Using an X-ray free electron laser (XFEL), we have previously determined room-temperature (RT) serial femtosecond crystallography (SFX) structures of the ferric and Compound I redox states of DtpB,26 a B-type member of the dye-decolorizing peroxidase (DyP) family. Such an approach results in “pristine” DtpB structures that do not exhibit the effects of X-ray-generated radiation damage. The RT-SFX DtpB ferric and Compound I structures revealed that the distal heme pocket, which is composed of an Asp–Arg–Asn triad, was void of H2O molecules. DtpB, therefore, represents an exemplar of a His–heme-ligated peroxidase in which the distal heme pocket favors a dry site. By disrupting the distal heme pocket Asp–Asn–Arg triad in DtpB, our RT-SFX structures reveal that a wet site can be formed.

To assess whether disruption of the Asp–Arg–Asn triad in DtpB leads to a wet distal heme pocket, microcrystals of each variant in the Fe(III)–heme state were produced and subjected to RT-SFX crystallography using a high viscosity extruder sample delivery system at the SACLA XFEL beamline BL2 EH3. For all variants, well-defined electron density peaks were present in the distal heme pocket, consistent with the presence of resident H2O molecules. In the D152A/N245A variant, H2O molecules are in identical spatial positions to the D152A variant, indicating that in the absence of the Asp–Asn dyad. the preferred spatial arrangement of the resident H2O molecules is the space vacated by the Asp152 side chain. In the D152A, D152A/N245A, and R243 variants, w1 is positioned close enough to the heme–Fe(III) to be a bonding interaction (average Fe(III)–OH2 distances within the DtpB hexamer assembly of 2.52, 2.83, and 2.28 Å, respectively). For the N245A variant, k1H aligns with values for the wild type (WT) and the D152A variant, with the double variant being an order of magnitude lower. Notably, the pH dependence of the double variant shows that the rates measured are an order of magnitude less than the single variants while still retaining linear dependencies on [H2O2]. These results indicate that the on-rate for H2O2 binding to Fe(III)–heme is much lower in the double variant, but the bound H2O2 behaves the same as in the single variants. The H2O network is identical in the double and D152A variant structures, so the reason for this lower rate constant of H2O2 binding must be a consequence of removing (or disrupting) the Asp–Asn dyad.

>MGGEVEEPEPQMVLSPLTSAAIFLVVTIDSGGEDTVRDLLSDVASLERAVGFRAQPDGRLSCVTGIGSEAWDRLFSGARPAGLHPFRELDGPVHRAVATPGDLLFHIRASRLDLCFALATEIMGRLRGAVTPQDEVHGFKYFDERDMLGFVAGTENPTGAAARRAVLVGAEDPAFAGGSYAVVQKYLHDIDAWEGLSVEAQERVIGRRKMTDVELSDDVKPADSHVALTSVTGPDGSDLEILRDAMPFGSVGREEFGTYFIGYARTPEVTETMLERMFLGTASAPHDRILDFSTAVTGSLFFTPAADFLEDLSARP[6x]>SNAMDYQTIPSQGLSGEICVPGDKSISHRAVLLAAIAEGQTQVDGFLMGADNLAMVSALQQMGASIQVIEDENILVVEGVGMTGLQAPPEALDCGNSGTAIRLLSGLLAGQPFNTVLTGDSSLQRRPMKRIIDPLTLMGAKIDSTGNVPPLKIYGNPRLTGIHYQLPMASAQVKSCLLLAGLYARGKTCITEPAPSRDHTERLLKHFHYTLQKDKQSICVSGGGKLKANDISIPGDISSAAFFIVAATITPGSAIRLCRVGVNPTRLGVINLLKMMGADIEVTHYTEKNEEPTADITVRHARLKGIDIPPDQVPLTIDEFPVLLIAAAVAQGKTVLRDAAELRVKETD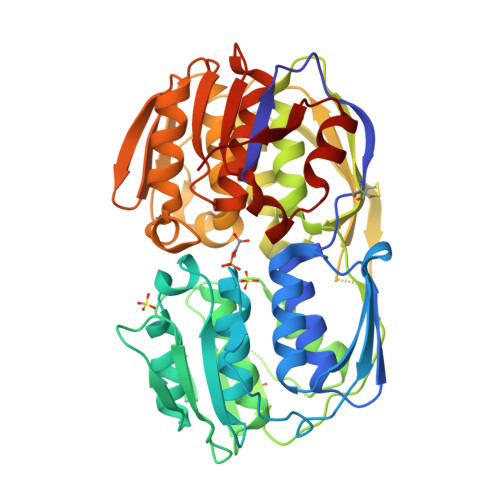RIAAMVDGLQKLGIAAESLPDGVIIQGGTLEGGEVNSYDDHRIAMAFAVAGTLAKGPVRIRNCDNVKTSFPNFVELANEVGMNVKGVRGRGGF[6x]> MSDQHDERRRFHRIAFDADSEILQGERRWEVLLHDVSLHGILVGQPQDWNGDPQRPFEARLYLGLDVLIRMEISLAWARDGLLGFE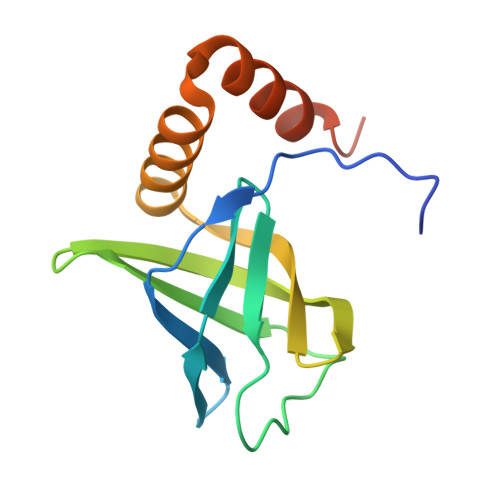CQHIDLDSISHLRRLVELNLGDEELLERELALLVSAHDDLEHHHHHH>[2x]MAHHHHHHSAALEVLFQGPGMAETKLQLFVKASEDGESVGHCPSCQRLFMVL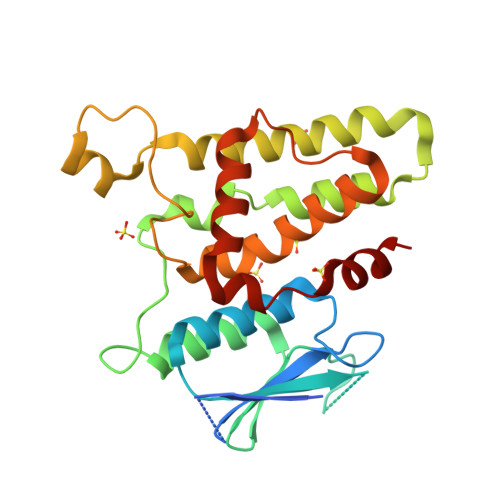LLKGVPFTLTTVDTRRSPDVLKDFAPGSQLPILLYDSDAKTDTLQIEDFLEETLGPPDFPSLAPRYRESNTAGNDVFHKFSAFIKNPVPAQDEALYQQLLRALARLDSYLRAPLEHELAGEPQLRESRRRFLDGDRLTLADCSLLPKLHIVDTVCAHFRQAPIPAELRGVRRYLDSAMQEKEFKYTCPHSAEILAAYR> MGSDSIDTPNYDVQKHINKLCGMLLITEDANHKFTGLIGMLYAMSRLGREDTIKILRDAGYHVKANGVDVTTHRQDINGKEMKFEVLTLASLTTEIQINIEIESRKSYKKMLKEMGEVAPEYRH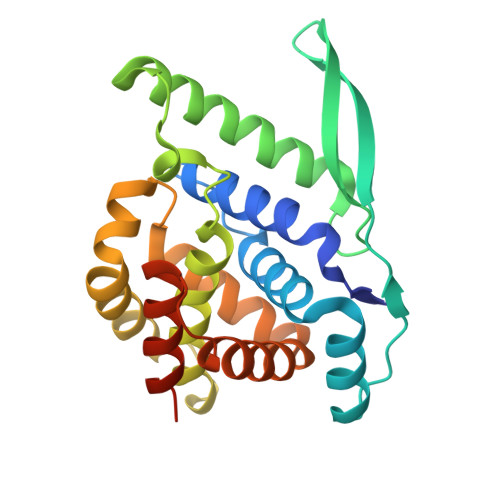DSPDCGMIILCIAALVITKLAAGDRSGLTAVIRRANNVLKNEMKRYKGLLPKDIANSFYEVFEKHPHFIDVFVHFGIAQSSTDGGSRVEGIFAGLFMNAYGLEHHHHHH>[2x]MSLSDIHQITPFLHIPDMQE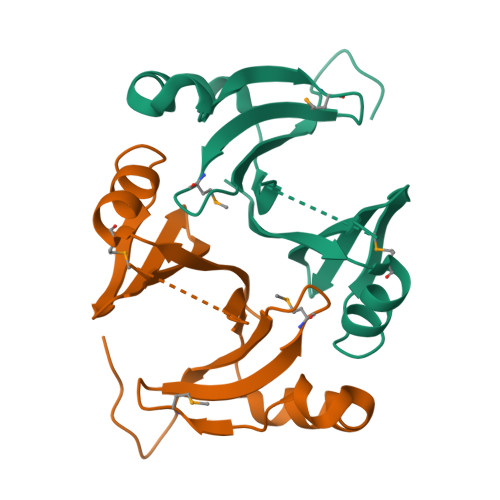ALTLFCDTLGFELKYRHSNYAYLELSGCGLRLLEEPARKIIPDGIARVAICIDVSDIDSLHTKLSPALENLPADQVEPLKNMPYGQREFQVRMPDGDWLNFTAPLAEGHHHHHH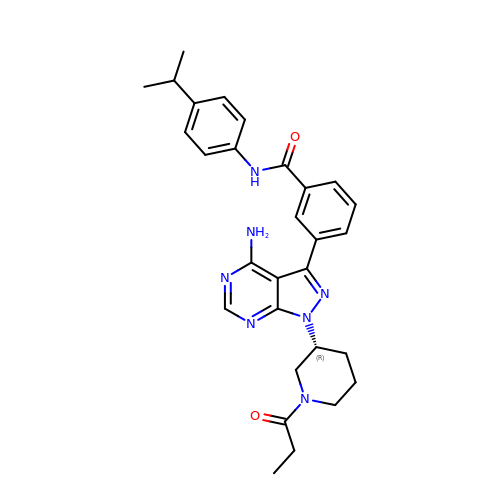3-{4-amino-1-[(3R)-1-propanoylpiperidin-3-yl]-1H-pyrazolo[3,4-d]pyrimidin-3-yl}-N-[4-(propan-2-yl)phenyl]benzamide | C29 H33 N7 O2 | OQUNLLPGZMGVNR-HSZRJFAPSA-N>MASNLVEMFNAALNWVTMILESPSARVVLFGVPIRGHFFVEGLLGVVIIILLTRKSYKPPKRPLTEQEIDELCDEWVPEPLIPPITEDMKHEPPVLESAAGPHTTVNGKDVVNFASANYLGLIGHEKLLESCTSALEKYGVGSCGPRGFYGTIDVHLDCETRISKFLGTPDSILYSYGLSTMFSTIPCFCKKGDVIVADEGVHWGIQNGLQLSRSTIVYFKHNDMESLRITLEKIMTKYKRSKNLRRYIVAEAVYQNSGQIAPLDEIVKLKEKYRFRVILDESNSFGVLGRSGRGLAEHHSVPIEKIDVVTAAMGHALATEGGFCTGNARIIDYQRLSSSGYVFSASLPPYLASAAITAIDVIDQNPDMLVKLKQNVALLWKGLSDIKGMSLTSNRESPIVFLKLEKSSGSAKDDLLLLEKMADRALKEDSLLVVSSKRSFLDKCRLPVGIKLYVSAGHSESDLLKASESLKRLASELLLKS[2x];>MITIPYLTAVSTYFSYGLLFAFGQLRDFFRRFIDWWFTSNLQGYAPICLGHEDFYIRRLYHRIQDCFERPISSAPDAWFDVVERYSNDNNKTLKRTTKTSRCLNLGSYNYLGFGSFDEYCTPRVIESLKKFSASTCSSRVDAGTTSVHAELEECVTRFVGKPAAVVFGMGYATNSAIIPVLIGKGGLIISDSLNHSSIVNGARGSGATIRVFQHNTPSHLERVLREQIAEGQPRTHRPWKKIIVVVEGIYSMEGEICHLPEVVAICKKYKAYVYLDEAHSIGAIGKTGKGICELLGVDTADVDVMMGTFTKSFGSCGGYIAGSKELIQYLKHQCPAHLYATSIPTPSAQQIISAIKVILGEDGSNRGAQKLARIRENSNFFRAELQKMGFEVLGDNDSPVMPIMLYNPAKIPAFSRECLRQKVAVVVVGFPATPLLLARARICISASHSREDLIRALKVISKVGDLSGIKYFPAEPKKIEQSKNDIKLD[2x];>[2x]MADYKDDDDKSGPDEVDASGRMNWVQRKIYLYNVTFGLYMLDWWERYLFNSLVVVLMWFVLYNGTRYFSELFQRHLT;>MANLYVKAVPPPDMNRNTEWFMYPGVWTTYMLILFFGWLVVLSVSGCSPGMAWTVVNLAHFVVTYHSFHWMKGTPFADDQGIYNGLTWWEQMDNGQQLTRNRKFLTLVPVVLYLIASHTTDYRHPWLFLNTLAVMVLVVAKFPNMHKVRIFGINGDK[2x]

The serine palmitoyltransferase (SPT) complex catalyzes the first and rate-limiting step in sphingolipid biosynthesis in all eukaryotes. ORM/ORMDL proteins are negative regulators of SPT that respond to cellular sphingolipid levels. We determined the cryo–electron microscopy structure of Arabidopsis SPT-ORM1 complex, composed of LCB1, LCB2a, SPTssa, and ORM1, in an inhibited state. The SPT-ORM1 complex is a ceramide sensor in the ER that controls cellular sphingolipid homeostasis.

Each protomer of the SPT-ORM1 dimer consists of LCB1, LCB2a, SPTssa, and ORM1 at a 1:1:1:1 ratio, and the transmembrane (TM) helix of LCB1 is swapped. In each protomer, a pyridoxal 5′-phosphate (PLP) cofactor was covalently linked to the ε-amino group of Lys311 in LCB2b as an internal aldimine. In addition, a robust lipid-like density that might belong to ceramide could be unambiguously resolved between ORM1 and LCB2a in the cytosolic membrane leaflet, which will be further discussed below. A ceramide molecule is sandwiched between ORM1 and LCB2a in the cytosolic membrane leaflet. The small polar head of C24-ceramide forms potential hydrogen bond interactions with the side-chain groups of Asn17 in ORM1 and Tyr55 in LCB2a and the main chain group of Ser67 in ORM1. The aliphatic sphingosine and acyl chains of ceramide are coordinated by numerous hydrophobic residues from both ORM1 and LCB2a. Unlike either of these, the N terminus of AtORM1 (residues 5 to 8) forms an antiparallel hybrid β sheet with the N terminus of LCB2a (residues 1 to 5) in the AtSPT-ORM1 complex structure. The potential acyl-CoA binding pocket in the AtSPT-ORM1 structure is partially shielded by Met14 and Asn15 from ORM1.> CGCAAT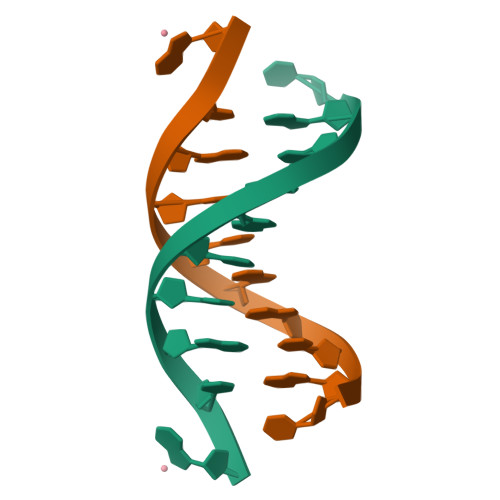TGCG> MGKSHSPVHWKSAAEIVELVKSKQISPREVVESTIDLIEQRDPGLNAVVYKAYDEAREKAAALERRIMQGEPVGMLAGVPTLMKDLFAAKPGWPSTLGGIRALKDARGAAGVWSTYPLKMSGEDSLLLGQTNSPVYGFRGTTDNTFFGPTRNPFNLDFNAGGSSGGAAALVADGIVPVAGGTDGGGSIRIPAAWT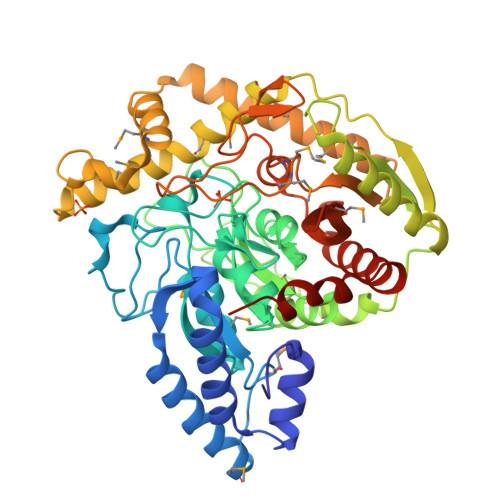NTYGFQPSIGRVPFKSRPNAFHPGPYLYEGPITRTVRDAALAMNVLHGFDRRDPASLRVKLDFTSALAQGVRGKKIGLTLNYGVFPVQQEIQDLIGKAARVFTELGAHVEFVDLGIPYSQKQMSDAWCRMIAIPTVASMQALRKEGIDLYGEHRADIPDALMKWIDAVADISVQQISADQLLRTTVFDCMNGVFDRFDLLLAPTLACMPVRNATDGCTEGPSQINGEEIDPLIGWCMTYLTNFSGHPSASVPAGLIDGLPAGMLIIGDRQADLDVIAASAAFERASPWSQYYDIPAGRPLHHHHHH> MMKTITLYLDPASLPALNQLMDFTQNNEDKTHPRIFGLSRFKIPDNIITQYQNIHFVELKDNRPTEALFTILDQYPGNIELNIHLNIAHSVQLIRPILAYRFKHLDRVSIQQLNLYDDGSMEYVDLEKEENKDISAEIKQAEKQLSHYLLTGKIKFDNPTIARYVWQSAFPVKYHFLSTD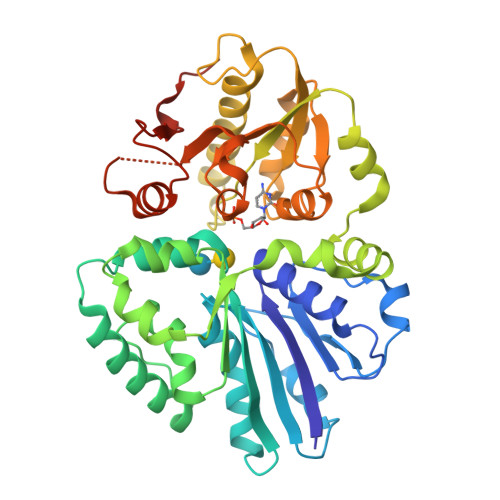YFEKAEFLQPLKEYLAENYQKMDWTAYQQLTPEQQAFYLTLVGFNDEVKQSLEVQQAKFIFTGTTTWEGNTDVREYYAQQQLNLLNHFTQAEGDLFIGDHYKIYFKGHPRGGEINDYILNNAKNITNIPANISFEVLMMTGLLPDKVGGVASSLYFSLPKEKISHIIFTSNKQVKSKEDALNNPYVKVMRRLGIIDESQVIFWDSLKQLGGGLEHHHHHH>[2x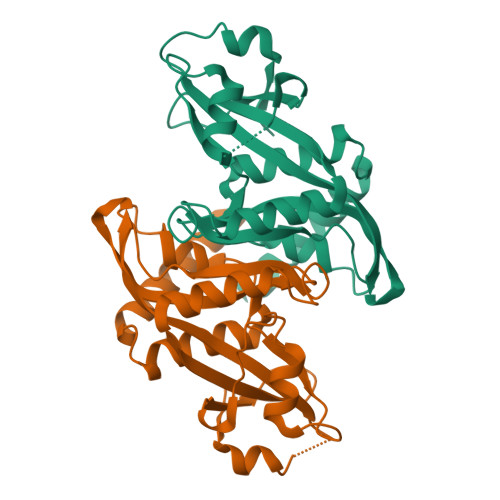]GMSTTTVPELKQISREEAMRLGPGWSHSCHAMLYAANPGQLFGRIPMRFSVLMQMRFDGLLGFPGGFVDRRFWSLEDGLNRVLGLGLGGLRLTEADYLSSHLTEGPHRVVAHLYARQLTLEQLHAVEISAVHSRDHGLEVLGLVRVPLYTQKDRVGGFPNFLSNAFVSTAKYQLLFALKVLNMMPSEKLAEALASATEKQKKALEKLLPPSS> MKVRVKAPCTSANLGVGFDVFGLCLKEPYDVIEVEAIDDKEIIIEVDDKNIPTDPDKNVAGIVAKKMIDDFNIGKGVKITIKKGVKAGSGLGSSAASSAGTAYAINELFKLNLDKLK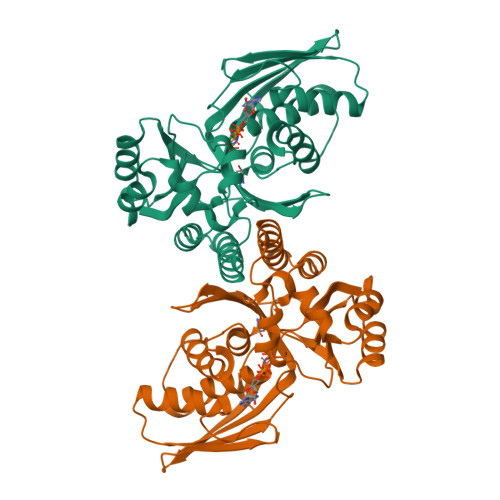LVDYASYGELASSGAKHADNVAPAIFGGFTMVTNYEPLEVLHIPIDFKLDILIAIPNISINTKEAREILPKAVGLKDLVNNVGKACGMVYALYNKDKSLFGRYMMSDKVIEPVRGKLIPNYFKIKEEVKDKVYGITISGSGPSIIAFPKEEFIDEVENILRDYYENTIRTEVGKGVEVV Zinc RING finger 3 (ZNRF3) and its homolog RING finger 43 (RNF43) are trans-membrane E3 ubiquitin ligases that negatively regulate Wnt signaling. ZNRF3 and RNF43 contain an extracellular N-terminal protease-associated (PA) domain, a single pass trans-membrane helix and an intracellular C-terminal RING domain with E3 ligase activity. Interaction of ZNRF3 or RNF43 with complexes of frizzled receptors (FZD) and low-density lipoprotein receptor-related protein (LRP) 5/6 leads to Frizzled ubiquitination and endocytosis of the heterodimeric receptors, thereby reducing the capacity of Wnt-driven signal transduction. RNF43 and its homolog ZNRF3 have been identified as E3 ligases that ubiquitinate Frizzled receptors for degradation, whereas RSPO1 captures ZNRF3 for removal from membrane, thereby increasing Frizzled expression on the cell surface.

We co-crystallized ZNRF3 ectodomain with RSPO1 consisting of the Fu1 and Fu2 domains. The ZNRF3-RSPO1 complex reveals an extensive interface, burying ~1,200 Å2, between the two molecules. The interaction site on RSPO1 is formed by the β-hairpins 1 and 2 of the Fu1 domain, which form an extended face that contacts ZNRF3. Apart from some side-chain rearrangements, no major conformational change is observed in ZNRF3 upon binding to RSPO1. Four copies of ZNRF3-RSPO1 are present in the asymmetric unit, which are arranged as a dimer of dimers. The dimeric arrangement observed in the structure of ZNRF3 is conserved in the crystal structure of ZNRF3-RSPO1; the two ZNRF3-RSPO1 dimers contact each other sideways through H-bond interactions made by the β1-β2 flaps of ZNRF3. In two copies of RSPO1 (denoted chains F and H) the Fu2 domains are less well packed and display higher B-factors than the other copies (chains E and G); these two sets differ by ~20° in Fu1-Fu2 domain orientations. Gln71 and Gly73 residues are located on the ZNRF3-RSPO1 interface and the Anonychia-related mutations, Q71R and G73R, would affect binding to ZNRF3 due to steric clashes and electrostatic repulsion. The structures of ZNRF3-RSPO1 and LGR5-RSPO1-RNF43 show that binding of ZNRF3 or RNF43 would disrupt the 2:2 LGR5-RSPO1 complex.

>[4x]GSKETAFVEVVLFESSPSGDYTTHTTGLTGRFSRAGAMLSAEGEIVQMHPLGLCNNNDEEDLYEYGWVGVVKLEQPELDPKPCLTVLGKAKRAVQRGATAVIFDVSENPEAIDQLNQGSEDPLKRPVVYVKGADAIKLMNIVNKQKVARARIQHLAAAHHHHHH;>GSRISAEGSQACAKGCELCSEVNGCLKCSPKLFILLERNDIRQVGVCLPSCPPGYFDARNPDMNKCIKCKIEHCEACFSHNFCTKCKEGLYLHKGRCYPACPEGSSAANGTMECSSPAAAHHHHHH[4x]>[2x]SVSSLLEVVADDLLKLNNNLKSLVGAENPVLVSAAEQIFGAGGKRLRPALVFLVSRATAELAGLLELTTEHQRLAEIIEMIHTASLIHDDVIDDSGMRRGKETIHQLYGTRVAVLAGDFMFAQSSWFLANLENIEVIKLISQVIKDFASGEIKQASTLFDCDITLDDYLLKSYYKTASLIAASTRSAAIFSGVSTAICEQMYEYGRNLGLSFQVVDDILDFTQSAEQLGKPAGSDLA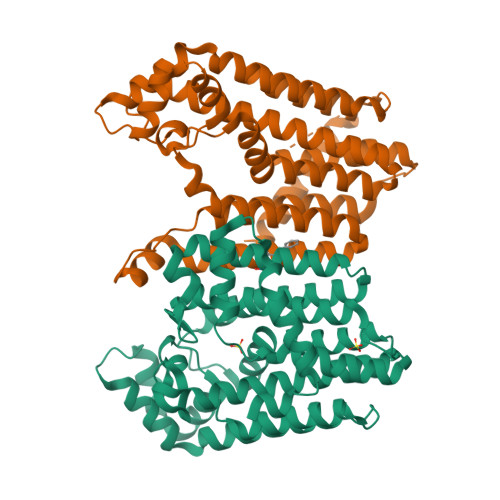KGNLTAPVIFALQDEPQLREIIDSEFSETNSLATAIELVHRSGGIKRAHELAREKGEIAIQSLQCLPRSEFRSTLENMVKYNLERID[(1R,2R)-2-(2-methoxybenzene-1-carbonyl)cyclopentyl]propanedioic acid | C16 H18 O6 | 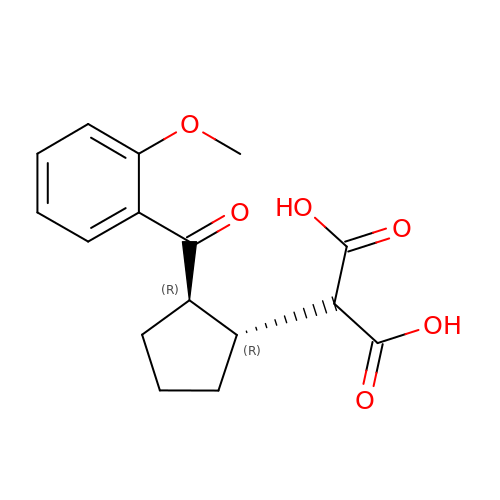KFADNUOGNGGPQM-QVDQXJPCSA-N>[2x]MATQAKRPRVAGPVDGGDLDPVACFLSWCRRVGLELSPKVAVSRQGTVAGYGMVARESVQAGELLFVVPRAALLSQHTCSIGGLLERERVALQSQSGWVPLLLAL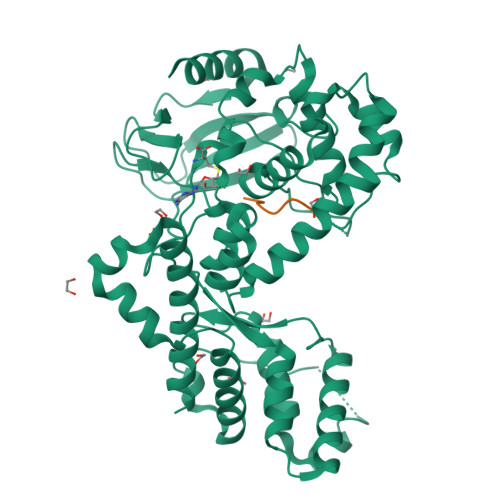LHELQAPASRWRPYFALWPELGRLEHPMFWPEEERRCLLQGTGVPEAVEKDLANIRSEYQSIVLPFMEAHPDLFSLRVRSLELYHQLVALVMAYSFQEPLEEEEDEKEPNSPVMVPAADILNHLANHNANLEYSANCLRMVATQPIPKGHEIFNTYGQMANWQLIHMYGFVEPYPDNTDDTADIQMVTVREAALQGTKTEAERHLVYERWDFLCKLEMVGEEGAFVIGREEVLTEEELTTTLKVLCMPAEEFRELKDQDGGGDDKREEGSLTITNIPKLKASWRQLLQNSVLLTLQTYATDLKTDQGLLSNKEVYAKLSWREQQALQVRYGQKMILHQLLELTS;>[2x]RKRTYETFKSIMKKS>[3x]ATCATAWSSSSVYTNGGTVSYNGRNYTAKWWTQNERPGTSDVWADKGACG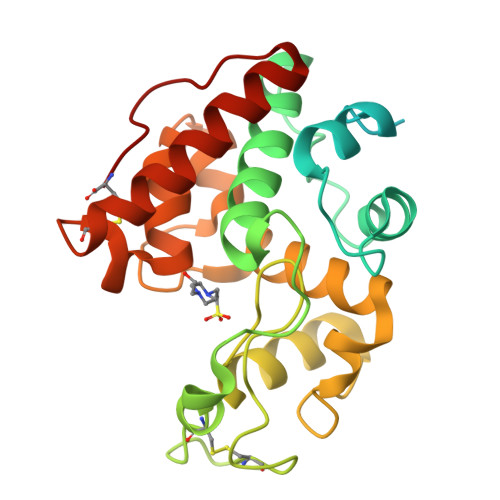TGGEGPGGNNGFVVSEAQFNQMFPNRNAFYTYKGLTDALSAYPAFAKTGSDEVKKREAAAFLANVSHETGGLFYIKEVNEANYPHYCDTTQSYGCPAGQAAYYGRGPIQLSWNFNYKAAGDALGINLLANPYLVEQDPAVAWKTGLWYWNSQNGPGTMTPHNAIVNNAGFGETIRSINGALECNGGNPAQVQSRINKFTQFTQILGTTTGPNLSC>[3x]MKRIGLTGNI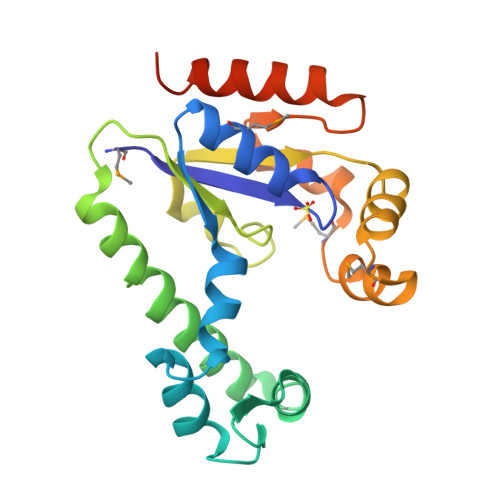GCGKSTVAQMFRELGAYVLDADKLIHSFYRKGHPVYEEVVKTFGKGILDEEGNIDRKKLADIVFKDEEKLRKLEEITHRALYKEIEKITKNLSEDTLFILEASLLVEKGTYKNYDKLIVVYAPYEVCKERAIKRGMSEEDFERRWKKQMPIEEKVKYADYVIDNSGSIEETYKQVKKVYEELTRDPLEHHHHHH>MGSTGNAEIQIIPTHSSDEEANLFAMQLASAAVLPMALKAAIELDVLEIMAKSVPPSGYISPAEIAAQLPTTNPEAPVMLDRVLRLLASYSVVTYT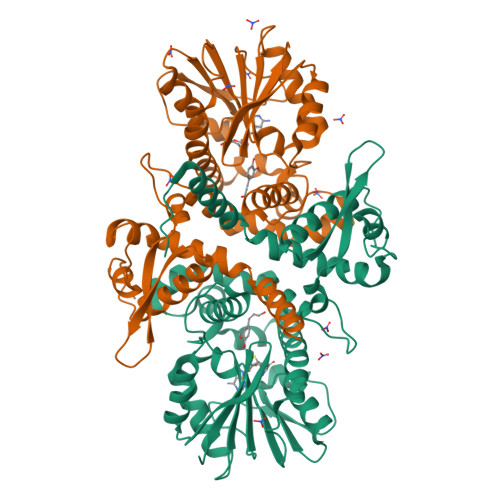LRELPSGKVERLYGLAPVCKFLTKNEDGVSLAPFLLLATDKVLLEPWFYLKDAILEGGIPFNKAYGMNIWDYFGTDHRINKVFNKGMSSNSTITMKKILEMYNGFEGLTTIVDVGGGTGAVASMIVAKYPSINAINFDLPHVIQDAPAFSGVEHLGGDMFDGVPKGDAIFIKWICHDWSDEHCLKLLKNCYAALPDHGKVIVAEYILPPSPDPSIATKVVIHTDALMLAYNPGGKERTEKEFQALAMASGFRGFKVASCAFNTYVMEFLKTA[4x]> GGSRGGYDRGGYRGRGGDRGGFRGGRGGGDRGGFGPGKM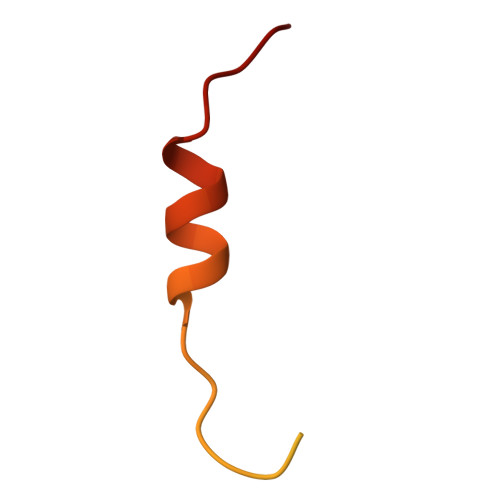DSRGEHRQDRRERLY Heterotrimeric kinesin-2 (KIF3/KAP3 in mammals) is one of the most widely expressed and abundant kinesins functioning as a complex of heterodimeric KIF3 motor (KIF3A/KIF3B or KIF3A/KIF3C) and the armadillo repeat (ARM)–containing adaptor KAP3 (16–18). Notably, the tumor suppressor protein adenomatous polyposis coli (APC) has been identified as a KIF3/KAP3 cargo involved in RNA and vehicle transport crucial for neurons, accounting for ~12% of KIF3-associated organelles. Here, we present high-resolution cryo–electron microscopy structures of the heterotrimeric kinesin-2 complex (KIF3A/KIF3B/KAP3) bound to the cargo protein APC. Our findings reveal a previously uncharacterized KIF3 tail hook-like motif, termed the “HAC” domain, which mediates binding to both KAP3 adaptor and APC cargo.

To this end, we assembled a tetrameric KIF3A/B tail/KAP3-APC complex using the validated KIF3/KAP3-binding ARM repeat region of APC and attempted single-particle cryo-EM reconstruction. Ultimately, we successfully reconstructed the structure of the core ARM repeats of APC in complex with ABK. The KIF3/KAP3 region in this map is highly consistent with the ABK map. Based on the cryo-EM and XL-MS results, we found unexpectedly that the C-terminal ARM repeats of APC bind KIF3/KAP3 specifically at the ABK interface 1 region. The ABKC interface primarily involves the βh-310-αB segment within the H-βh-H of KIF3A, which contributes 11 residues, and the C-terminal helix of KAP3, which engages three residues, collectively interacting with 17 residues of the APCARM. Within this interface, the 310-αB region of KIF3A plays a central role, with Val624, Ala625, and Tyr626 from the 310-helix inserting into a hydrophobic pocket formed at the C-terminal region of APCARM. The KAP3 C-terminal helix also participates in the interaction of APCARM, with Gln682 and Met686 engaging APCARM. As the αB region within the KIF3A H-βh-H domain was not fully built in the final map, we incorporated the KIF3A tail–linking loop region from the docking model for further MD-based free energy calculations. These calculations revealed that the KIF3A-APCARM interaction contributes the dominant binding energy—approximately three times greater than that of the KAP3-APCARM interaction—while KIF3B showed no contribution to APCARM binding. The structural alignment of the HAC regions in KIF3A and KIF3B reveals that the presence of Pro616 in KIF3B induces a loop reorientation following the β-hairpin and prevents the formation of the αB helix after the 310-helix. The wild-type kinesin-2 complex exhibited a strong binding affinity to APCARM, with a dissociation constant (KD) of 34.7 ± 0.6 nM.

> MGSSHHHHHHSQSLQEEAQGKTKKLKKVWTMLMAAKSEMADLQQEHQREIEGLLENIRQLSRELRLQMLIIDNFIPQDYQEMIENYVHWNEDIGEWQLKCVAYTGNNMRKQTPVPDKKERDPFEVDLSHVYLAYTEESLRQSLMKLERPRTSKGKARPKMGRRKRSAKPETVIDSLLQ;> MSLQQEVDIKTKKLKKLFSKLQAVKAEIHDLQEEHIKERQELEQTQNELTRELKLKHLIIENFIPLEEKNKIMNRSFFDDEEDHWKLHPITRLENQQMMKRPVSAVGYKRPLSQHARMSMMIRPEPRYRAENIMLLELDMPSRTTRDYEGPAISPKVQAALDAALQDEDEIQVDASSFESTASRKPKARPKSGRKSGSSSSSSGNPASQFYPQSRGLVPK;> MQGEDARYLKRKVKGGNIDVHPSEKALIVQYEVEATILGEMGDPMLGERKECQKIIRLKSLNANTDITSLARKVVEECKLIHPSKLSEVEQLLYYLQNRRDSLPGKEKKEKSSKPKDPPPFEGMEIDEVANINDMDEYIELLYEDIPDKVRGSALILQLARNPDNLEELLLNETALGALARVLREDWKQSVELATNIIYIFFCFSSFSHFHGLITHYKIGALCMNIIDHELKRHELWQEELSKKKKAVDEDLENQTLRKDYDKTFKKYQGLVVKQEQLLRVALYLLLNLAEDTRTELKMRNKNIVHMLVKALDRDNFELLILVVSFLKKLSIFMENKNDMVEMDIVEKLVKMIPCEHEDLLNITLRLLLNLSFDTGLRNKMVQVGLLPKLTALLGNENYKQIAMCVLYHISMDDRFKSMFAYTDCIPQLMKMLFECSDERIDLELISFCINLAANKRNVQLICEGNGLKMLMKRALKLKDPLLMKMIRNISQHDGPTKNLFIDYVGDLAAQISSDEEEEFVIECLGTLANLTIPDLDWELVLKEYKLVPFLKDKLKPGAAEDDLVLEVVIMIGTVSMDDSCAALLAKSGIIPALIELLNAQQEDDEFVCQIIYVFYQMVFHQATRDVIIKETQAPAYLIDLMHDKNNEIRKVCDNTLDIIAEYDEEWAKKIQSEKFRWHNSQWLEMVESRQLD;> MHHHHHHSQDSCISMRQSGCLPLLIQLLHGNDKDSVLLGNSRGSKEARARASAALHNIIHSQPDDKRGRREIRVLHLLEQIRAYCETCWEWQEAHEQGMDQDKNPMPAPVEHQICPAVCVLMKLSFDEEHRHAMNELGGLQAIAELLQVDCEMYGLTNDHYSVTLRRYAGMALTNLTFGDVANKATLCSMKGCMRALVAQLKSESEDLQQVIASVLRNLSWRADVNSKKTLREVGSVKALMECALEVKKESTLKSVLSALWNLSAHCTENKADICAVDGALAFLVGTLTYRSQTNTLAIIESGGGILRNVSSLIATNEDHRQILRENNCLQTLLQHLKSHSLTIVSNACGTLWNLSARNPKDQEALWDMGAVSMLKNLIHSKHKMIAMGSAAALRNLMANRPAKYKDANIMSPGSSLPSLHVRKQKALEAELDAQHLSETFDNIDNLSPKASHRSKQRHKQNLYGDYAFDANRHDDSRSDNFNTGNMTVLSPYLNTTVLPSSSSSRGSLDSSRSEKDRSLERERGIGLSAYHPTTENAGTSSKRGLQITTTAAQIAKVMEEVSAIHTSQDDRSSASTTEFHCVADDRSAARRSSASHTHSNTYNFTKSENSNRTCSMPYAKVEYKRSSNDSLNSVTSSDGYGKRGQMKPSVESYSEDDESKFCSYGQYPADLAHKIHSAN>[4x]SMGQETSYIEDNCNQNGAISLIFSLKEE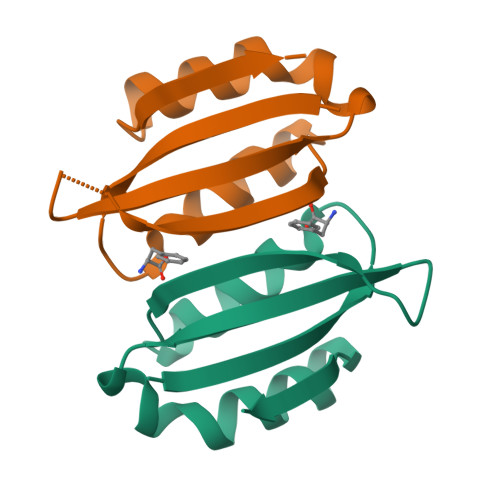VGALAKVLRLFEENDVNLTHIESRPSRLKKDEYEFFTHLDKRSLPALTNIIKILRHDIGATVHELSRDKKKDTV>ESMELACPAERSGHVAVSDGRHMFVWGGYKSNQVRGLYDFYLPREELWIYNMETGRWKKINTEGDVPPSMSGSCAVCVDRVLYLFGGHHSRGNTNKFYMLDSRSTDRVLQWERIDCQGIPPSSKDKLGVWVYKNKLIFFGGYGYLPEDKVLGTFEFDETSFWNSSHPRGWNDHVHILDTETFTWSQPITTGKAPSPRAAHACATVGNRGFVFGGRYRDARMNDLHYLNLDTWEWNELIPQGICPVGRSWHSLTPVSSDHLFLFGGFTTDKQPLSDAWTYCISKNEWIQFNHPYTEKPRLWHTACASDEGEVIVFGGCANNLLVHHRAAHSNEILIFSVQPK[2x]

As a substrate receptor subunit of the CUL2-RBX1 E3 complex, KLHDC2 features a KELCH-repeat propeller domain, which can recognize the di-glycine C-end degron of its substrates with a nanomolar affinity. We set out to identify compounds that can anchor to the diglycine-binding site of KLHDC2, which has recently been suggested as a promising PROTACs E3 platform for targeted protein degradation.

Out of these, 29 compounds were successfully synthesized and characterized in an AlphaLISA competition assay, in which each compound was tested for its ability to compete with a diglycine-containing SelK C-end degron peptide for binding KLHDC2. While several compounds showed detectable activity in displacing the degron peptide, compound 29 (C29) stood out with the best IC50 of ~ 3 μM. To reveal the binding mode of compound 29, we soaked the crystals of apo KLHDC2 with the compound and determined the structure of the KLHDC2-C29 complex at 2.0 Å resolution. The triazole moiety next to the carboxyl group of the compound is nestled among three aromatic residues (Tyr163, Trp191, and Trp270) and stabilized by a NH…N hydrogen bond. The interaction of the compound with the E3 is further strengthened by a hydrogen bond formed between Lys147 and the central carbonyl group of the small molecule as well as direct packing of the tert-butylphenyl group to the auxiliary chamber of the degron-binding pocket. In contrast to the two ends of the compound, the dimethyl-sulfide linker in the middle of the compound shows poor electron density, indicating higher structural flexibility. Overall, the binding mode of compound 29 is highly similar to that of the diglycine C-end degron with a binding pose closely matching the prediction. Finally, a high resolution X-ray crystallographic structure validates the predicted docking pose for the KLHDC2 ligand complex, demonstrating the effectiveness of our method in lead discovery.> MEKDGLCRADQQYECVAEIGEGAYGKVFKARDLKNGGRFVALKRVRVQTGEEGMPLSTIREVAVLRHLETFEHPNVVRLFDVCTVSRTDRETKLTLVFEHVDQDLTTYLDKVPEPGVPTETIKDMMFQLLRGLDFLHSHRVVHRDLKPQNILVTSSGQIKLADFGLARIYSFQMALTSVVVTLWYRAPEVLLQSSYATPVDLWSVGCIFAEMFRRKPLFRGSSDVDQLGKILDVIGLPGEEDWPRDVALPRQAFHSKSAQPIEKFVTDIDELGKDLLLKCLTFNPAKRISAYSALSHPYF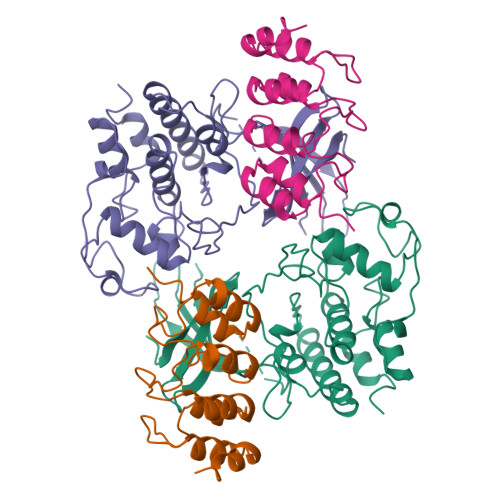QDLERCKENLDSHLPPSQNTSELNTA;> MEPAAGSSMEPSADWLATAAARGRVEEVRALLEAGANPNAPNSYGRRPIQVMMMGSARVAELLLLHGAEPNCADPATLTRPVHDAAREGFLDTLVVLHRAGARLDVRDAWGRLPVDLAEELGHRDVARYLRAAAGGTRGSNHARIDAAEGPSDIPD> SMANTITASVIHPMLHQNTSTFSEQRFSSTFTGEEFFLADHVVKGQRVLPGVAYLEMARSAMEHAVGEDVHGNTSMKLQNVIWARPIVVGDQPVRVHTGLVLEEDGEVSYQIYSEAEGSDAEIVVHSQGNAVLTPRSELHMLDLPVLQEQCSEQVISSEEFYEFFSAIQIDYGSGHKGIDKVYVGPGQVLAKLILPLSVTGSVDQFVLHPSLMDSALQASVELTLSSRHVMSSDSLAKRKPVMPFALEEMEIIRPCTSEMWAYVRYSDGSQAGNKVEKYDIDLCDDI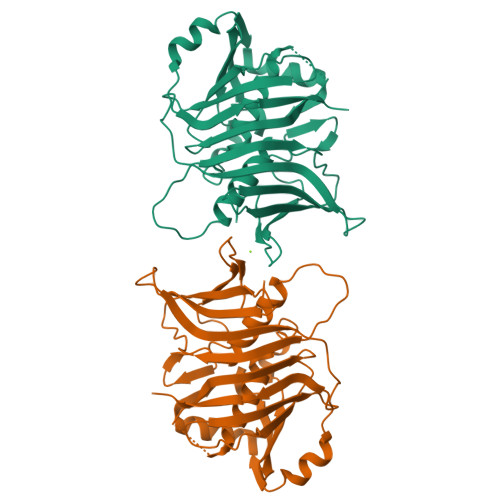GTICVRMKGFTSRVLEREIQTDRTAAKGAVETAS> MYEGNNMRSMMGTSYEDSRLNKRTEL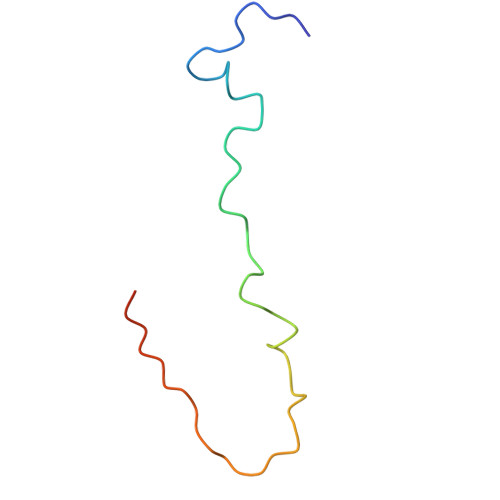NENMSIDTNKSEDSYGVQIHSLSKQSFTGDVEEE> GGGGSMGKEQKEKKDGNLSIKEEVEKELNKKSTAELFRKIKNEKISFFLPFKCLPAQHRKLLFISFVCAVLSGGTLPFFISVFGVILKNMNLGDDINPIILSLVSIGLVQFILSMISSYCMDVITSKILKTLKLEYLRSVFYQDGQFHDNNPGSKLRSDLDFYLEQVSSGIGTKFITIFTYASSFLGLYIWSLIKNARLTLCITCVFPLIYVCGVICNKKVKLNKKTSLLYNNNTMSIIEEALMGIRTVASYCGEKTILNKFNLSETFYSKYILKANFVEALHIGLINGLILVSYAFGFWYGTRIIINSATNQYPNNDFNGASVISILLGVLISMFMLTIILPNITEYMKALEATNSLYEIINRKPLVENNDDGETLPNIKKIEFKNVRFHYDTRKDVEIYKDLSFTLKEGKTYAFVGESGCGKSTILKLIERLYDPTEGDIIVNDSHNLKDINLKWWRSKIGVVSQDPLLFSNSIKNNIKYSLYSLKDLEAMENYYEEN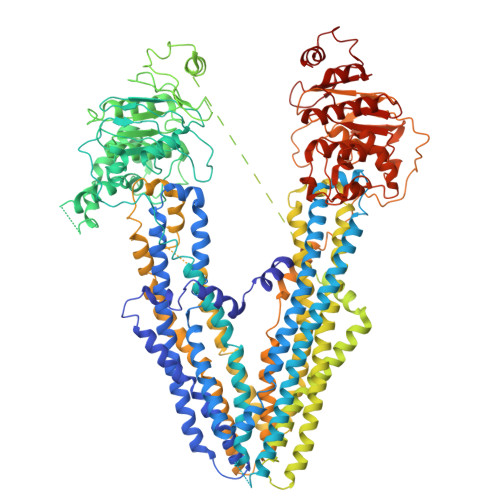TNDTYENKNFSLISNSMTSNELLEMKKEYQTIKDSDVVDVSKKVLIHDFVSSLPDKYDTLVGSNASKLSGGQKQRISIARAIMRNPKILILDEATSSLDNKSEYLVQKTINNLKGNENRITIIIAHRLSTIRYANTIFVLSNRERSDNNNNNNNDDNNNNNNNNNNKINNEGSYIIEQGTHDSLMKNKNGIYHLMINNQKISSNKSSNNGNDNGSDNKSSAYKDSDTGNDADNMNSLSIHENENISNNRNCKNTAENEKEEKVPFFKRMFRRKKKAPNNLRIIYKEIFSYKKDVTIIFFSILVAGGLYPVFALLYARYVSTLFDFANLEYNSNKYSIYILLIAIAMFISETLKNYYNNKIGEKVEKTMKRRLFENILYQEMSFFDQDKNTPGVLSAHINRDVHLLKTGLVNNIVIFSHFIMLFLVSMVMSFYFCPIVAAVLTFIYFINMRVFAVRARLTKSKEIEKKENMSSGVFAFSSDDEMFKDPSFLIQEAFYNMHTVINYGLEDYFCNLIEKAIDYKNKGQKRRIIVNAALWGFSQSAQLFINSFAYWFGSFLIKRGTILVDDFMKSLFTFIFTGSYAGKLMSLKGDSENAKLSFEKYYPLMIRKSNIDVRDDGGIRINKNLIKGKVDIKDVNFRYISRPNVPIYKNLSFTCDSKKTTAIVGETGSGKSTFMNLLLRFYDLKNDHIILKNDMTNFQDYQNNNNNSLVLKNVNEFSNQSGSAEDYTVFNNNGEILLDDINICDYNLRDLRNLFSIVSQEPMLFNMSIYENIKFGREDATLEDVKRVSKFAAIDEFIESLPNKYDTNVGPYGKSLSGGQKQRIAIARALLREPKILLLDEATSSLDSNSEKLIEKTIVDIKDKADKTIITIAHRIASIKRSDKIVVFNNPDRNGTFVQSHGTHDELLSAQDGIYKKYVKLAK> MIIPALDLIGGTVVRVVRLHQGDYARQRDYGNDPLPRLQDYAAQGAGVLHLVDLTGAKDPAKRQIPLIKTLVAGVNVPVQVGGGVRTEEDVAALLKAGVARVVIASTAVKSPDVVKGWFERFGAQALVLALDVRIDEHGTKQVAVSGWQENSGVSLEQLVETYLPVGLKHVLCTDISRDGTLAGSNVSLYE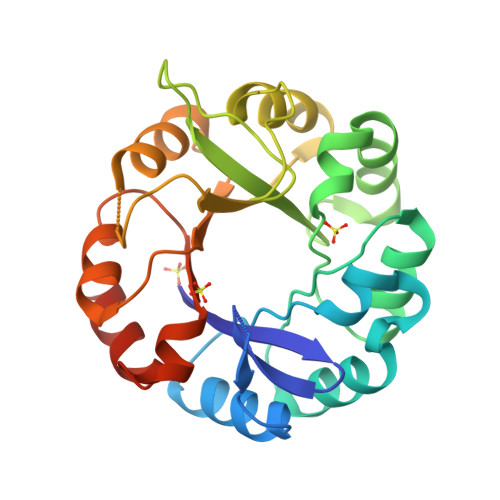EVCARYPQIAFQSSGGIGDIDDIAALRGTGVRGVIVGRALLEGKFTVKEAIQCWQNVKGHHHHHH>[3x]GSHMASMRVLLAPMEGVLDSLVRELLTEVNDYDLCITEFVRVVDQLLPVKVFHRICPELQNAS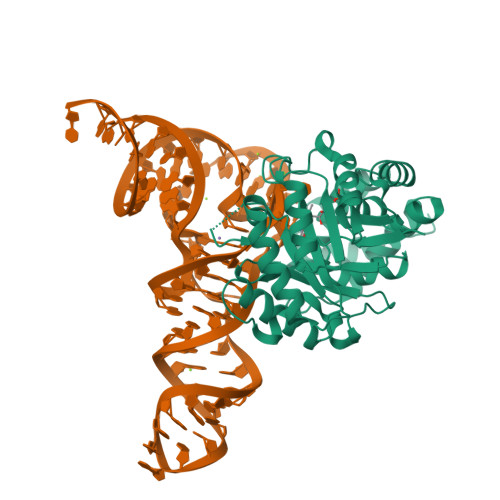RTPSGTLVRVQLLGQFPQWLAENAARAVELGSWGVDLNCGAPSKTVNGSGGGATLLKDPELIYQGAKAMREAVPAHLPVSVKVRLGWDSGEKKFEIADAVQQAGATELVVHGRTKEQGYRAEHIDWQAIGDIRQRLNIPVIANGEIWDWQSAQQCMAISGCDAVMIGRGALNIPNLSRVVKYNEPRMPWPEVVALLQKYTRLEKQGDTGLYHVARIKQWLSYLRKEYDEATELFQHVRVLNNSPDIARAIQAIDIEKL2-KETO,5-NITRO,6-HYDROXY-3,5-HEXADIENOIC 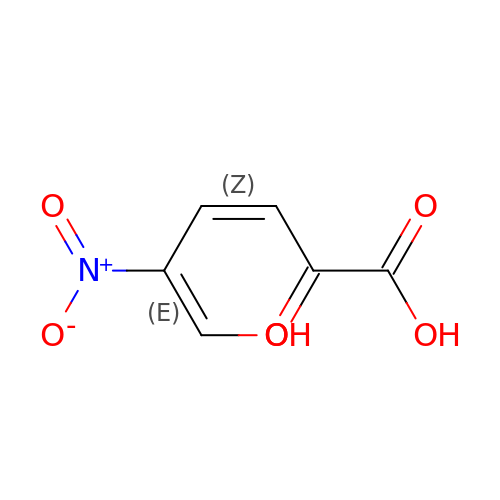ACID | C6 H5 N O6 | UDOBAQIWFWMQMT-BXTBVDPRSA-N> MGSSHHHHHHGTGSYITSLYKKAGWMGSNEAQVKKESIGEIMGKLMQGEIGDEELSKRIKEIFGKRLQWGYKPTHQQQLAFNLDFIKSLKEMDMSGEIDTMNEETYELPSAFLEAAFGKTIKQSGCYFKDETTTIDEAEEASHELYCERAQIKDGQTVLDIGCGQGGLVLHIAQKYKNCHVTGLTNSKAQKNYILMQAEKLQLSNVDVILADVTKHESDKTYDRILVIATIEHMKNIQLFMKKLSTWMTEDSLLFVDHICHKTFSHHFEAIDEDDWYSGFIFPKGCVTILSASALLYFQDDVTILDHWVVNGMHMARSVDAWRKKLDKNMELAREILLPGLGSKEAVNGVITHIRTFCMGGYEQFSYNNGEEWMVAQML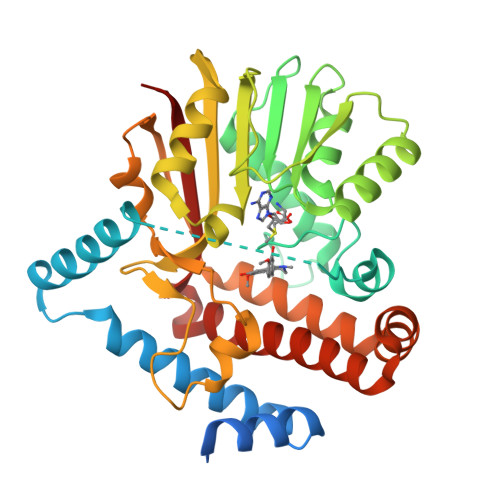FKKK In this study, we investigate AfuABC (Actinobacillus ferric uptake ABC), a BPDT originally identified as an iron-specific transporter in Actinobacillus pleuropneumoniae, a Gram-negative upper respiratory tract pathogen. The locus afuABC encodes 3 polypeptides corresponding to a conventional BPDT–AfuA (a periplasmic binding protein or PBP), AfuB (an inner membrane permease), and AfuC (a cytosolic ATPase). AfuA is a class II/cluster D periplasmic binding protein with two globular α/β domains linked by a dual β-stranded hinge. Instead, AfuABC is a trio of proteins that bind and transport sugar-phosphates such as glucose-6-phosphate (G6P).

A subsequent ligand screen by ITC with structurally similar molecules revealed that three other sugar-phosphates including fructose-6-phosphate (F6P), sedoheptulose-7-phosphate (S7P) and M6P had affinities of 8, 57 and 960 nM respectively for AfuA. Structures of AfuA bound to F6P (2.0Å) and S7P (1.3Å) were also solved to confirm ligand coordination. Similar to the G6P structure, both F6P and S7P were found in the β-anomer conformation. Between the three holo-AfuA structures, strand and amino acid placement and conformation were identical (RMSD < 0.4Å between Cα chains). F6P binding affinities of the single site AfuA mutants displayed the same trend as for G6P, suggesting a similar binding mechanism between the two ligands. Our observation that both furan (F6P and S7P) and pyran (G6P) ligands could bind AfuA suggests the position of hydroxyl determinants is more important than steric fitting of the overall ring structure into the binding pocket. On the opposing end of the pocket, redundant phosphate-coordinating residues such as Ser37 cooperate to hold the phosphate moiety of ligands. This bipartite binding cleft is able to discriminate between isomers of the same sugar-phosphate (G6P vs. G1P) and between differing orientations of side chains around the carbohydrate ring (F6P vs. R5P).

>[4x]GSKGRLVIYCSATNVMCENAAKTFEQKYDVKTSFIRNGSGSTFAKIEAEKNNPQADVWYGGTLDPQSQAGELGLLEAYRSPNIDQIMPKFQDPAKVKGNLSSAVYIGILGFAVNTERLKKLGIEKIPQCWNDLTDPKLKGEIQIADPQSSGTAYTAIATFAQLWGEDKAFDYFKHLHPNISQYTKSGITPARNAARGETTVGIGFLHDYALEKEQGAPLEMVVPCEGTGYELGGVSILKGARNLDNAKLFVDFALSKEGQETAWKKGQALQTLTNTTAEQSPLAFDLTKLKLIDYDFEKYGASDERKRLINKWVDEIKLAK> MMAEHDQNNDEYKFAELDSYDMDQAGESDLDSEASYQSGKEGLTKKKDIKRNALIAIGAVVFIMVMYKIIGWMFFSDKSSQVTSKPAIPPVTQVATPQPVQTIPTTTPIQQVQPTTIIEDDPDLKKKVSAIEMTQQSLRSEVNALSEQINAVNNNIKNLNAQIVNLNQIIGNMSNQIARQSEVINVLMARTTPKKVVKVSRPIVQARIIYYIQAVIPGRAWLIGSNGSTLTVREGSKIPGYGMVKLIDSLQGR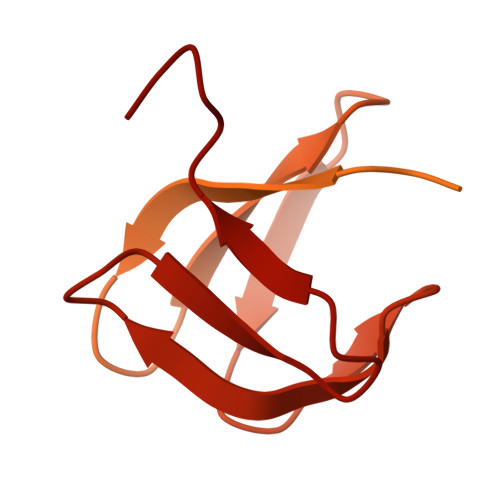ILTSSGQVIKFSQEDS>[2x]MFIKPGRCPKPAVQEDFDAARYLGVWYDIQRLPNKFQKGECATATYS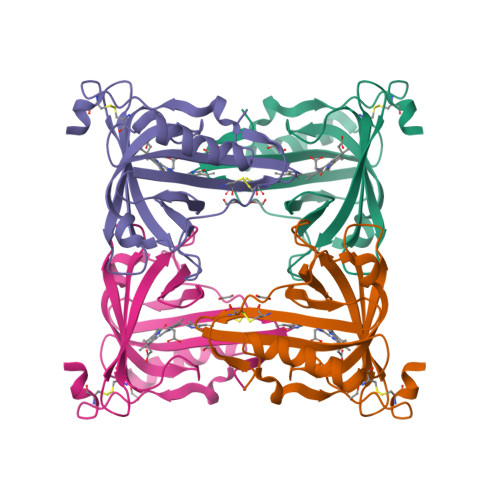LSPGVGFSVFNRERLANGTIKSVIGSAIAEDPCEPAKLQFFHENAAPVPYWVLSTDYDNYALVYSCINLGASHAAYASIVSRQPTLPEETIKKLQGTMSSFGVGVDTLLTTNQDAAYCSAMNQKLAAALEHHHHHH> SVQQASRSKVSVAPLHLESAKEPPLNTYKPKEPFTATIVSVESLVGPKAPGETCHIVIDHGGNVPYWEGQSYGVIPPGENPKKPGAPQNVRLYSIASTRYGDNFDGRTGSLCVRRAVYYDPETGKEDPSKNGVCSNFLCNSKPGDKIQLTGPSGKIMLLPEEDPNATHIMIATGTGVAPFRGYLRRMFMEDVPNYRFGGLAWLFLGVANSDSLLYDEEFTSYLKQYPDNFRYDKALSREQKNRSGGKMYVQDKIEEYSDEIFKLLDG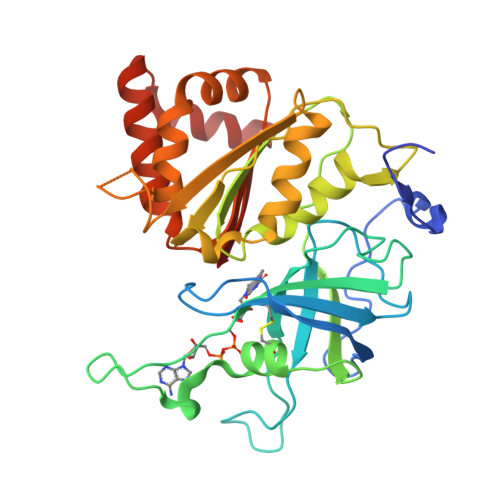GAHIYFCGLKGMMPGIQDTLKKVAERRGESWDQKLAQLKKNKQWHVEVY Bifunctional N-deacetylase-N-sulfotransferase (NDST) enzymes are the first to act on nascent heparosan after its polymerization, converting GlcNAc sugars to GlcNS, via deacetylated glucosamine (GlcN) intermediates. NDST1 is a Golgi lumen resident type-II transmembrane protein, which contains a single pass N-terminal helix that anchors the catalytic luminal portions of the enzyme to the Golgi membrane. We have carried out a detailed structural and functional characterization of NDST1, the dominant human NDST isoform, revealing a 3-domain architecture consisting of a non-catalytic NTD, in addition to catalytic deacetylase and sulfotransferase domains. A distinctive feature of the NDST1 protein architecture is the opposing orientation of its catalytic deacetylase and sulfotransferase domains, which effectively precludes a simple substrate transfer mechanism for bifunctionality.

To better understand the molecular basis for NDST1 activity, and how it is modulated by nAb binding, we sought to resolve three-dimensional structures of NDST1 and its complexes with nAb7 and nAb13. A cryo-EM volume of NDST1 alone was calculated to a nominal resolution of 2.70 Å (Relion Au-FSC = 0.143), with the resulting map of sufficient quality to model nearly all residues along the protein chain, using the AlphaFold2 model as a starting point for refinement. Disulfide bonds between C586–C601 and C818–C828 were clearly visible in the cryo-EM density, with the former at lower occupancy, possibly due to its surface location being susceptible to reduction by 1 mM DTT, present in the sample buffer. We observed unambiguous density within the sulfotransferase active site corresponding to a molecule of 5’-phosphoadenosine-3’-phosphate (PAP; present in the cryo-EM sample), which binds NDST1 via H-bonds and salt bridges to K614–T618, R782, K833, R835, Y837, R782 and W817, as well as a π-stacking interaction from adenine to F816. The C828–D841 loop at the mouth of the PAP site partially occludes the ligand from solvent, suggesting a role as a stabilizing lid that encloses PAP(S) after its engagement with the sulfotransferase domain. Clear density, distinct from surrounding protein sidechains, was visible at the center of this triad, consistent with Ca2+ coordinated to H389, H393, D320, although a full coordination sphere could not be resolved, possibly due to local disorder within the open catalytic cleft. Further density within the deacetylase active site was tentatively modeled as a second Ca2+, consistent with the presence of multiple divalent ions in the active site of Agd3 and other deacetylases. The NDST1 NTD adopts a Rossman-like fold, comprising a central layer of β-sheets flanked by α-helices on each side, although disorder prevented modeling of loops K171–S179, S191–D197, V215–W225 and K242–L262.

> SRTDPLVLVFVESLYSQLGQEVVAILESSRFKYRTEIAPGKGDMPTLTDKGRGRFALIIYENILKYVNLDAWNRELLDKYCVAYGVGIIGFFKANENSLLSAQLKGFPLFLHSNLGLKDCSINPKSPLLYVTRPSEVEKGVLPGEDWTVFQSNHSTYEPVLLAKTRSSESIPHLGADAGLHAALHATVVQDLGLHDGIQRVLFGNNLNFWLHKLVFVDAVAFLTGKRLSLPLDRYILVDIDDIFVGKEGTRMKVEDVKALFDTQNELRAHIPNFTFNLGYSGKFFHTGTNAEDAGDDLLLSYVKEFWWFPHMWSHMQPHLFHNQSVLAEQMALNKKFAVEHGIPTDMGYAVAPHHSGVYPVHVQLYEAWKQVWSIRVTSTEEYPHLKPARYRRGFIHNGIMVLPRQTCGLFTHTIFYNEYPGGSSELDKIINGGELFLTVLLNPISIFMTHLSNYGNDRLGLYTFKHLVRFLHSWTNLRLQTLPPVQLAQKYFQIFSEEKDPLWQDPCEDKRHKDIWSKEKTCDRFPKLLIIGPQKTGTTALYLFLGMHPDLSSNYPSSETFEEIQFFNGHNYHKGIDWYMEFFPIPSNTTSDFYFEKSANYFDSEVAPRRAAALLPKAKVLTILINPADRAYSWYQHQRAHDDPVALKYTFHEVITAGSDASSKLRALQNRCLVPGWYATHIERWLSAYHANQILVLDGKLLRTEPAKVMDMVQKFLGVTNTIDYHKTLAFDPKKGFWCQLLEGGKTKCLGKSKGRKYPEMDLDSRAFLKDYYRDHNIELSKLLYKMGQTLPTWLREDLQNTR3-bromo-5-(2H-tetrazol-5-yl)pyridine | C6 H4 Br N5 | 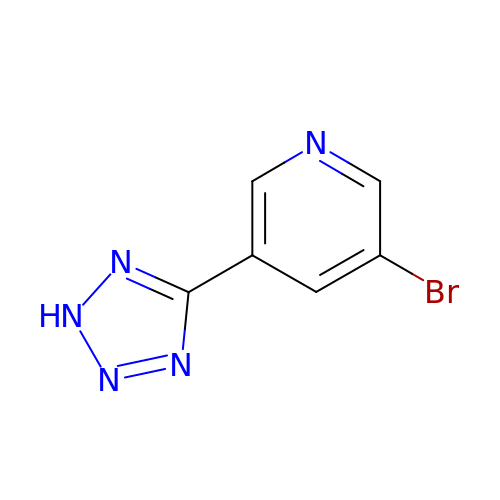XJGDASCALCDOQH-UHFFFAOYSA-N> SCLGSIMNPKSLTRGPRDKPTPLEELLPHAIEFINQYYGSFKEAKIEEHLARLEAVTKEIETTGTYQLTLDELIFATKMAWRNAPRCIGRIQWSNLQVFDARNCSTAQEMFQHICRHILYATNNGNIRSAITVFPQRSDGKHDFRLWNSQLIRYAGYQMPDGTIRGDAATLEFTQLCIDLGWKPRYGRFDVLPLVLQADGQDPEVFEIPPDLVLEVTMEHPKYEWFQELGLKWYALPAVANMLLEVGGLEFPACPFNGWYMGTEIGVRDFCDTQRYNILEEVGRRMGLETHTLASLWKDRAVTEINVAVLHSFQKQNVTIMDHHTASESF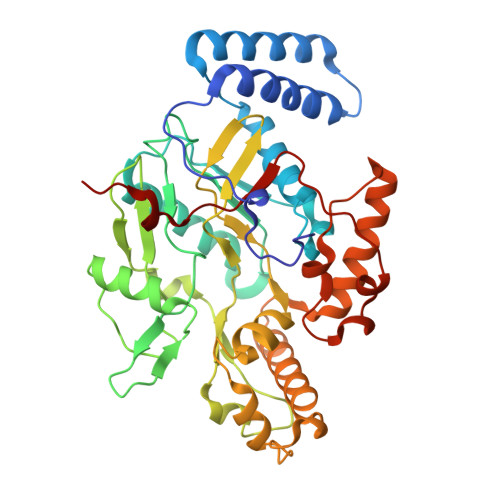MKHMQNEYRARGGCPADWIWLVPPVSGSITPVFHQEMLNYVLSPFYYYQIEPWKTHIWQ>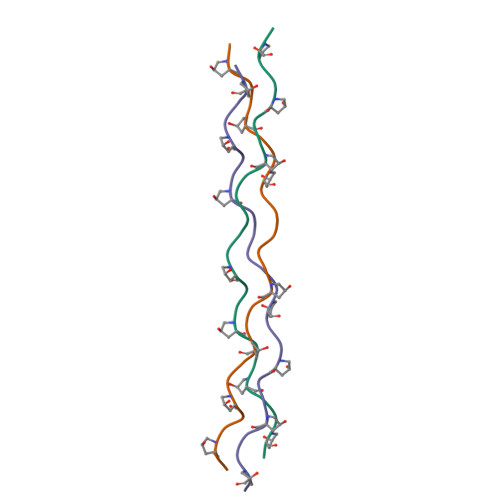[3x]XPPGPPGPPGPKGEPGPPGPPGPPGX>[2x]MSARISLFAVVVEDMAKSLEFYRKLGVEIPAEADSAPHTEAVLDGGIRLAWDTVETVRSYDPEWQAPTGGHRFAIAFEFPDTA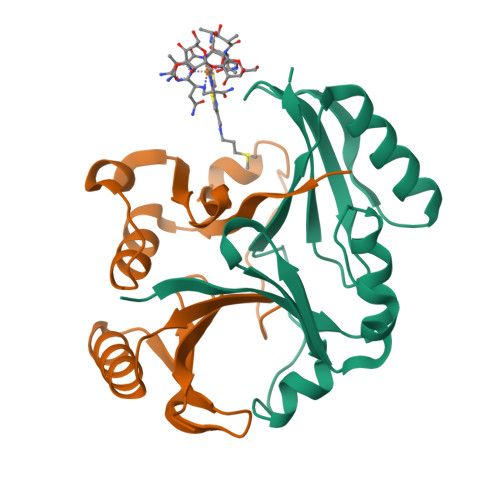SVDKKYAELVDAGYEGHLKPWNAVWGQRYAIVKDPDGNVVDLFAPLPLEHHHHHH> GA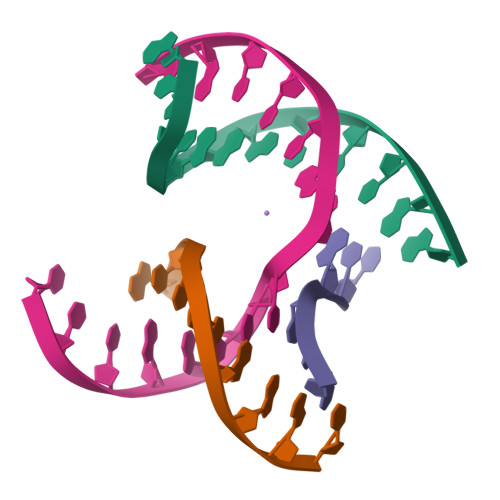GCAGACTTGA;> CGAGACTCA;> TCATCG;> TCTGAGTCAGTCTGC> 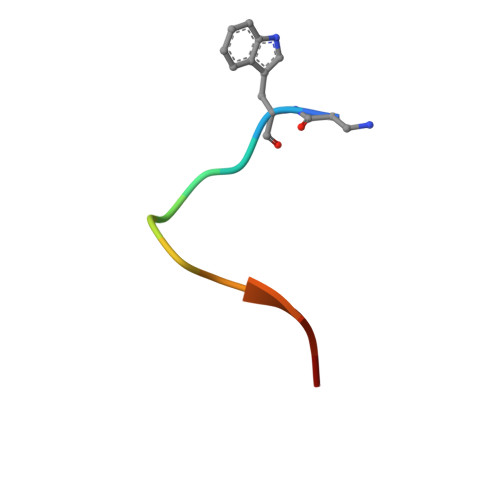XWLAYPDSVPYX>GPLGSLTMGAQDTLPVAAAFTETVNAYFKGADPSKCIVKITGEMVLSFPAGITRHFANNPSPAALTFRVINFSRLEHVLP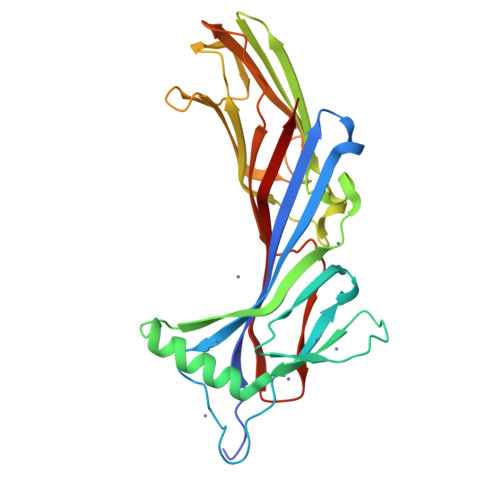NPQLLCCDNTQNDANTKEFWVNMPNLMTHLKKVSEQKPQATYYNVDMLKYQVSAQGIQSTPLNLAVNWRCEPSSTDLRIDYKYNTDAMTTAVALNNVQFLVPIDGGVTKLQAVLPPAVWNAEQQRILWKIPDISQKSENGGVGSLLARFQLSEGPSKPSPLVVQFTSEGSTLSGCDIELVGAGYRFSLIKKRFAAGKYLADN[2x]Rad53, and its mammalian ortholog the checkpoint kinase 2 (Chk2), are key effector kinases of the DNA replication checkpoint. Rad53 contains two forkhead-associated (FHA) domains, as well as two SQ/TQ cluster domains (SCD), flanking its kinase domain. The phosphoepitope-binding site recognizes an epitope present in DDK24, whereas one of the lateral surfaces of FHA1 interacts with the modified BRCT domain of Dbf416, herein referred to as HBRCT domain due to the presence of an additional α-helix at the N-terminus of the domain. We generated chimeras expressing the HBRCT (Dbf4) and FHA1 (Rad53) domains in tandem and solved the crystal structures of these chimeras in the absence and presence of a phosphorylated epitope derived from Cdc7.

Since we have previously shown that a peptide derived from this motif of Cdc7 (pPEP, 480DGESpTDEDDVVS491) binds to the FHA1 domain of Rad53 in a phosphorylation-dependent manner in vitro, we used this peptide for subsequent crystallographic studies. Crystals of the ternary Rad53-Dbf4-Cdc7 complex grew in the P21 space group and diffracted X-rays beyond 2.3 Å resolution. Similar to other structures of FHA1 domains bound to phosphorylated peptides, pPEP is bound at one end of the FHA1 domain and interacts with residues in the β3/β4, β4/β5 and β6/β7 loops. The phosphate moiety of pThr484 is held in place through hydrogen bonds with Arg70, Ser85, Asn86 and Thr106; the pT + 3 aspartate residue (Asp487) is anchored through a salt bridge with Arg83; and the main chain of the intervening residues is further stabilized through hydrogen-bonds with the main chain carbonyl of Ser82 and the side chain of Asn107. The Dbf4:Rad53 interface is similar, but not identical, to the binary complex. Binding of the phosphopeptide, however, induces a small rigid body movement of Dbf4 around the two interfaces holding the complex. The HBRCT domain seesaws pushing helix α1 away from the FHA1 domain while pulling the α0/β1 loop towards the FHA1 domain. Upon binding to pPEP, the side-chain of Lys118 (interface I in Dbf4) comes close to the side-chains of Asp123 (Dbf4) and Asp149 (Rad53) stabilizing the interaction of the C-terminus of helix α0 in Dbf4 with Rad53. On the ternary complex, Lys200 (interface II in Dbf4) is not hydrogen-bonded to Asn112. Binding to pPEP pushes the α3/β4 loop of Dbf4 closer to the β10 strand where the new conformation of Lys200 is stabilized through hydrogen bonds with Gln126 and Asp128.

>SHMTPKELLEWQTNWKKIMKRDSRIYFDITDDVEMNTYNKSKMDKRRDLLKRGFLTLGAQITQFFDTTVTIVITRRSVENIYLLKDTDILSRAKKNYMKVWSYEKAARFLKNLDVDLDHVDGSKFSQEQIGENIVCRVICTTGQIPIRDLSADISQVLKEKRSIKKVWTFGRNPACDYHLGNISRLSNKHFQILLGEDGNLLLNDISTNGTWLNGQKVEKNSNQLLSQGDEITVGVGVESDILSLVIFINDKFKQCLEQNKVDR[2x];>[2x]DGESTDEDDVVS Growth/differentiation factors 8 and 11 (GDF8/myostatin and GDF11/BMP11, respectively) are two closely related members of the activin/inhibin subclass that share ~90% sequence identity in their mature, C-terminal signaling domains and ~52% identity in their N-terminal prodomains. Similar to other TGFβ ligands, GDF8 and GDF11 are disulfide-linked dimers that are initially synthesized as precursors, which are cleaved by furin-like proteases to separate the N-terminal prodomain from the C-terminal mature domain. The ligand dimer elicits signal transduction by symmetrically binding two type II and two type I transmembrane serine/threonine kinase receptors. Similar to other ligands in the activin/inhibin subclass, GDF8 and GDF11 predominantly signal through the type II receptors, activin receptor kinase IIA (ActRIIA; ACVR2A) and ActRIIB (ACVR2B) and the type I receptors, activin-like receptor kinase 4 (ALK4; ACVR1B) and ALK5 (TβRI).

We resolved the structure of apo-GDF8 to 2.25 Å and the apo-GDF11 structure to 1.90 Å using X-ray crystallography, thus allowing a direct comparison to the recently published apo-GDF11 structure (middle). Our new apo-GDF11 structure, solved under similar crystallization conditions as apo-GDF8, adopted an exaggerated “open” conformation such that the fingers extend past the horizontal plane. This conformation shares a similar exaggerated “open” conformation to the crystal structure of GDF8 bound to a neutralizing antibody (bottom). However, the wrist region in our apo-GDF11 structure is also disordered and not resolved in the crystal structure, similar to apo-GDF8 (bottom). The previously published apo-GDF11 crystal structure adopts the classic “open” conformation with an ordered wrist helix that includes the additional interchain hydrogen bond between Q62A and the pre-helix loop observed in the FS288-bound GDF11 crystal structure. Interestingly and despite the high sequence identity, nearly identical crystallization conditions resulted in two distinct conformations. Although these conformations may be a result of the crystallization process, it supports the idea that GDF8 and GDF11 are flexible enough to be trapped in alternate states. Taken together, crystallization of both GDF8 and GDF11 in their apo states reveals intrinsic structural flexibility in these ligands.

>NLGLDCDEHSSESRCCRYPLTVDFEAFGWDWIIAPKRYKANYCSGQCEYMFMQKYPHTHLVQQANPRGSAGPCCTPTKMSPINMLYFNDKQQIIYGKIPGMVVDRCGCS[2x]>[4x]HNMKAFLDELKAENIKKFLYNFTQIPHLAGTEQNFQLAKQIQSQWKEFGLDSVELAHYDVLLSY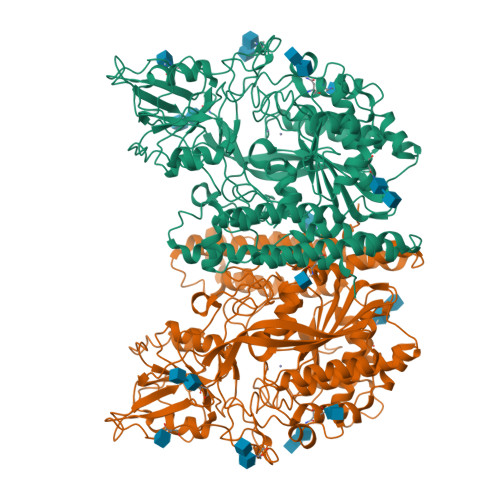PNKTHPNYISIINEDGNEIFNTSLFEPPPPGYENVSDIVPPFSAFSPQGMPEGDLVYVNYARTEDFFKLERDMKINCSGKIVIARYGKVFRGNKVKNAQLAGAKGVILYSDPADYFAPGVKSYPDGWNLPGGGVQRGNILNLNGAGDPLTPGYPANEYAYRRGIAEAVGLPSIPVHPIGYYDAQKLLEKMGGSAPPDSSWRGSLKVPYNVGPGFTGNFSTQKVKMHIHSTNEVTRIYNVIGTLRGAVEPDRYVILGGHRDSWVFGGIDPQSGAAVVHEIVRSFGTLKKEGWRPRRTILFASWDAEEFGLLGSTEWAEENSRLLQERGVAYINADSSIEGNYTLRVDCTPLMYSLVHNLTKELKSPDEGFEGKSLYESWTKKSPSPEFSGMPRISKLGSGNDFEVFFQRLGIASGRARYTKNWETNKFSGYPLYHSVYETYELVEKFYDPMFKYHLTVAQVRGGMVFELANSIVLPFDCRDYAVVLRKYADKIYSISMKHPQEMKTYSVSFDSLFSAVKNFTEIASKFSERLQDFDKSNPIVLRMMNDQLMFLERAFIDPLGLPDRPFYRHVIYAPSSHNKYAGESFPGIYDALFDIESKVDPSKAWGEVKRQIYVAAFTVQAAAETLSEVA>GIDPFTSQNTETKATIARKGEGSVLEQIDQGSILKLPSNLLFENATSDAINQDMMLYIERIAKIIQKLPKRVHINVRGFTDDTPLVKTRFKSHYELAANRAYRVMKVLIQYGVNPNQLSFSSYGSTNPIAPNDSLENRMKNNRV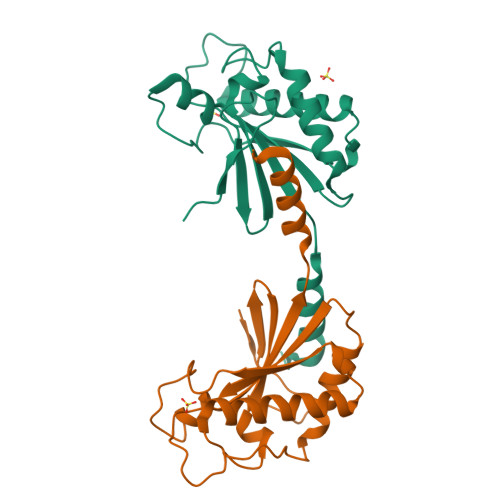EIFFSTDANDLSKIHSILDNEFNPHKQQE[4x]> GEIIGGTECKPHSRPYMAYLEIVTSNGPSKFCGGFLIRRNFVLTAAHCAGRSITVTLGAHNITEEEDTWQKLEVIKQFRH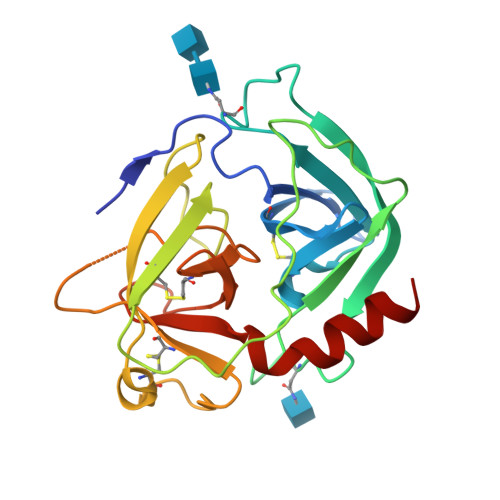PKYNTSTLHHDIMLLKLKEKASLTLAVGTLPFPSQFNFVPPGRMCRVAGWGRTGVLKPGSDTLQEVKLRLMDPQACSHFRDFDHNLQLCVGNPRKTKSAFKGDSGGPLLCAGVAQGIVSYGRSDAKPPAVFTRISHYRPWINQILQAN>[4x]GADDVVDSSKSFVMENFSSYHGTKPGYVDSIQKGIQKPKSGTQGNYDDDWKEFYSTDNKYDAAGYSVDNENPLSGKAGGVVKVTYPGLTKVLALKVDNAETIKKELGLSLTEPLMEQVGTEEFIKRFGDGASRVVLSLPFAEGSSSVEYINNWEQAKALSVELEINFETRGKRGQDAMYEYMAQACAGNRVRRSVGSSLSCINLDWDVIRDKTKTKIESLKEHGPIKNKMSESPNKTVSEEKAKQYLEEFHQTALEHPELSELKTVTGTNPVFAGANYAAWAVNVAQVIDSETADNLEKTTAALSILPGIGSVMGIADGAVHHNTEEIVAQSIALSSLMVAQAIPLVGELVDIGFAAYNFVESIINLFQVVHNSYNRPAYSPGHKTQPFLHDGYAVSWNTVEDSIIRTGFQGESGHD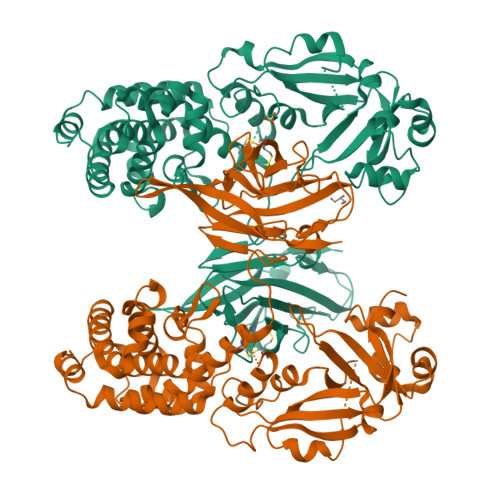IKITAENTPLPIAGVLLPTIPGKLDVNKSKTHISVNGRKIRMRCRAIDGDVTFCRPKSPVYVGNGVHANLHVAFHRSSSEKIHSNEISSDSIGVLGYQKTVDHTKVNSKLSLFFEIKS> SFPEVVELNVGGQVYFTRHSTLI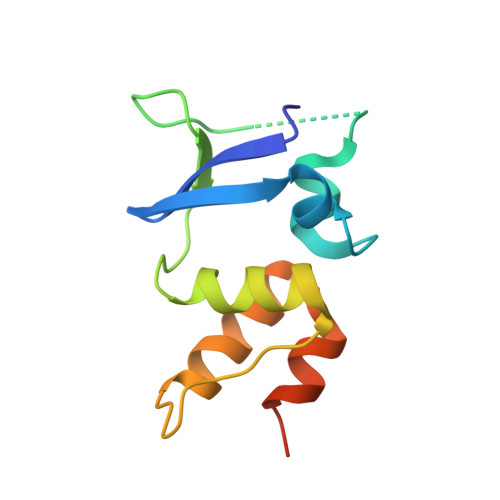SIPHSLLWKMFSPKRDTANDLAKDSKGRFFIDRDGFLFRYILDYLRDRQVVLPDHFPEKGRLKREAEYFQLPDLVKLLTPDEIKQSPDEF> MKRILVVDDEPNIRELLKEELQEEGY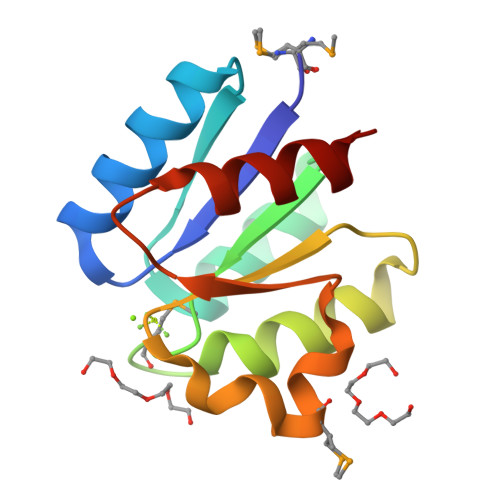EIDTAENGEEALKKFFSGNYDLVILDIEMPGISGLEVAGEIRKKKKDAKIILLTAYSHYRSDMSSWAADEYVVKSFNFDELKEKVKKLLS>[2x]SQLKSDRRFQLLAAAERLFAERGFLAVRLEDIGAAAGVSGPAIY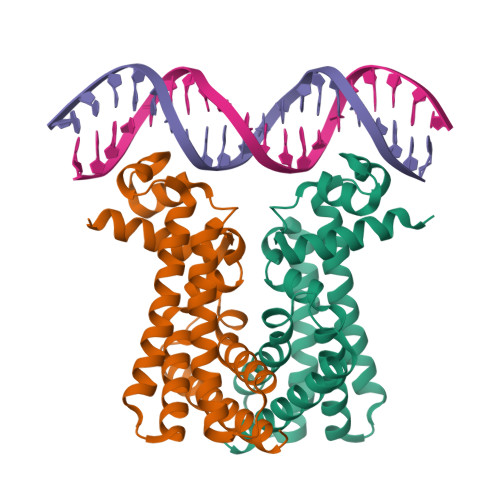RHFPNKESLLVELLVGVSARLLAGARDVTTRSANLAAALDGLIEFHLDFALGEADLIRIQDRDLAHLPAVAERQVRKAQRQYVEVWVGVLRELNPGLAEADARLMAHAVFGLLNSTPHSMKAADSKPARTVRARAVLRAMTVAALSAADRCL> EDPEVLFKNKGCVACHAIDTKKVGPAYAD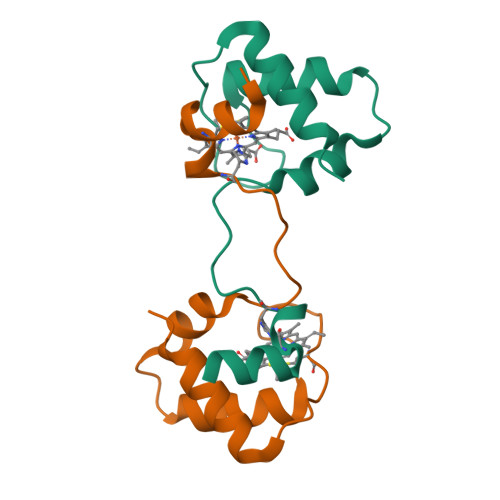VAKKYAGRKDAVDYLAGKIKKGGSGVWGSVPMPPQNVTDAEAKQLAQWILSIK;> NEQLAKQKGCMACHDLKAKMVGPAYKDVAAKFAGQAGAEAELAQRIKNGSQGVWGPIPMPPNAVSDDEAQTLAKWVLSQK(2E,4E,6Z,8E)-8-[3-cyclopropyl-2-(3-methylbutyl)cyclohex-2-en-1-ylidene]-3,7-dimethylocta-2,4,6-trienoic 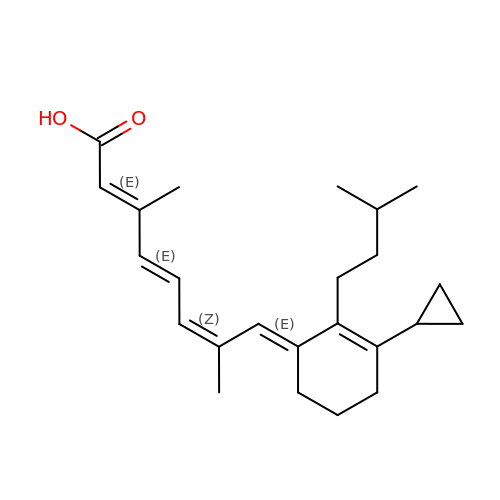acid | C24 H34 O2 | SCCVQQDOUFNKGM-RBEOCVBDSA-N>[2x]GPM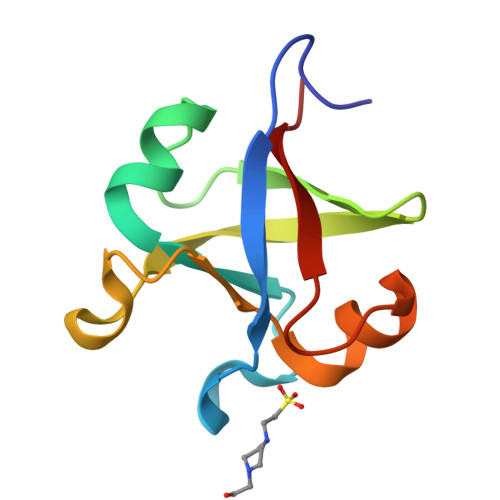PGLSVKLRVAEAYPEDVGKRIVRMDKASRAKLGVSVGDYVEVKKVKSVVARVAEAYPEDVGKGIVRMDKYERAKLGVSVGDYVEVKKVE>[2x]SNAMHSDALSWGHGPRLFEVFLEPTCPFSVKAFFKLDDLLAQAGEDNVTVRIR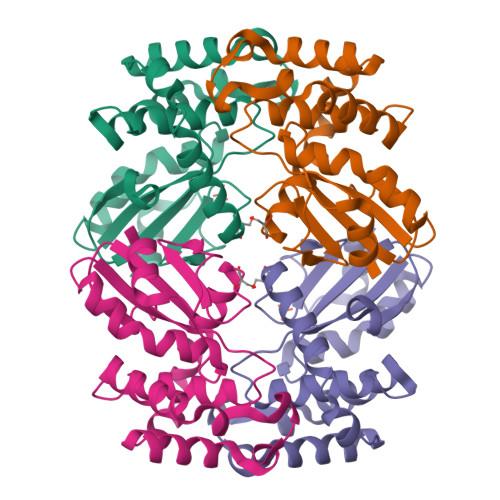LQSQPWHMFSGVIVRCILAAATLEGGKESAKAVMTAVASHREEFEFEHHAGGPNLDATPNDIIARIERYSGLALAEAFANPELEHAVKWHTKYARQNGIHVSPTFMINGLVQPGMSSGDPVSKWVSDIG>MAHHHH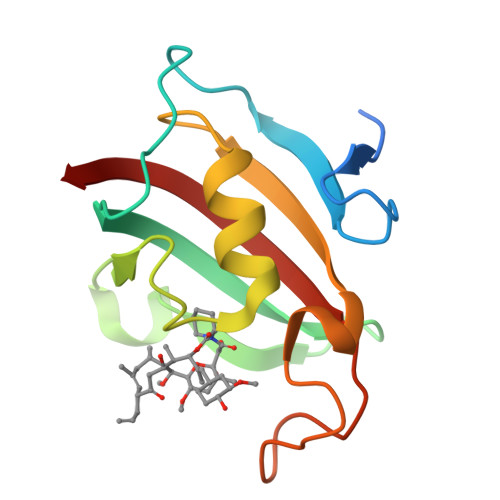HHMSTDWIPISQDQRLKKKIITAGSSDEQPPIGSKVSVHYTGTLTSGKKFDSSLDRGQPFVFTLGKGEVIRGWDLGVKSMKKGEKSYFEIPSDYAYGNNAIPGLIPANSTLMFEIELLSWK[4x]> MAGSSFSGKYQLQSQENFEAFMKAIGLPEELIQKGKDIKGVSEIVQNGKHFKFTITAGSKVIQNEFTVGEECELETMTGEKVKTVVQLEGDNKLVTTFKNI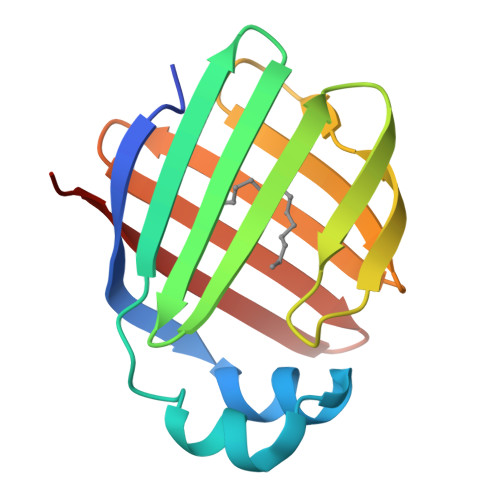KSVTELNGDIITNTMTLGDIVFKRISKRIGT> GMSLANQIDQFLGTIMQFAENKHEILLGKSESDVKLTSTQEHILMLLAEQISTNAKIAEKLKISPAAVTKALKKLQEQELIKSSRATNDERVVLWSLTE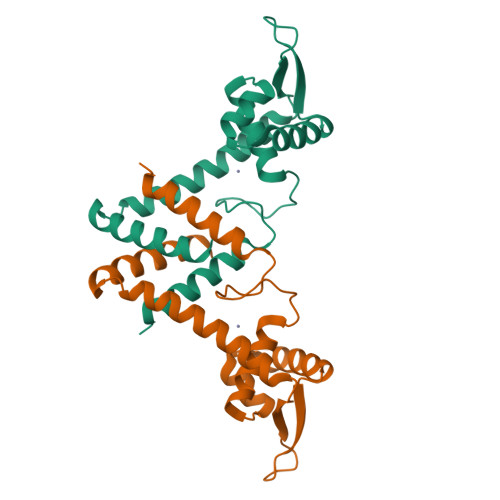KAVPVAKEHATHHEKTLSTYQELGNKFTDEEQEVISKFLSALTEEFQ> MSLGVLRYTLRARGHPNVTAGHRTTFEVTVDPEIGETADCIIGVSSSDSISTLPDEMKRAIARESSLVRVILRTENGYDEIRGYGHPELTLDHPTDIVCRKSDYICSRTLMIR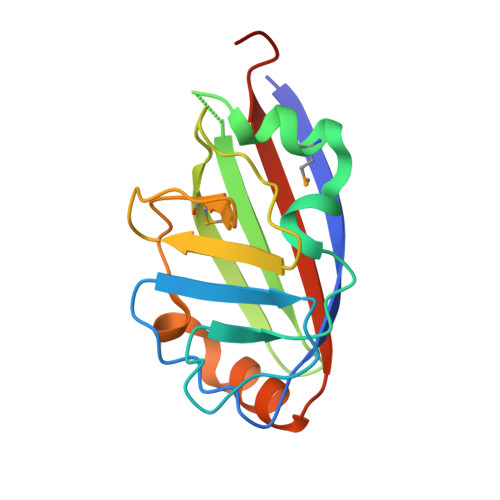ADKAAFDLDENLVRDLRKGRELKVEIIVEYEGHHHHHH(3~{R})-2-[(5-chloranylpyridin-2-yl)methyl]-3-(4-chlorophenyl)-4-fluoranyl-3-[[1-(hydroxymethyl)cyclopropyl]methoxy]-6-(2-oxidanylpropan-2-yl)isoindol-1-one | C28 H27 Cl2 F N2 O4 | 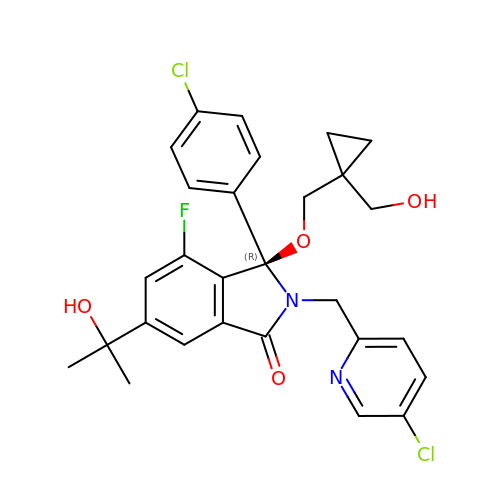WLOCTJJGJPSXJZ-MUUNZHRXSA-N>MSIISTKYLLQDAQANGYAVPAFNIHNAETIQAILEVCSEMRSPVILAGTPGTFKHIALEEIYALCSAYSTTYNMPLALHLDHHESLDDIRRKVHAGVRSAMIDGSHFPFAENVKLVKSVVDFCHSQDCSVEAELGRLGGVEDDMSVDAESAFL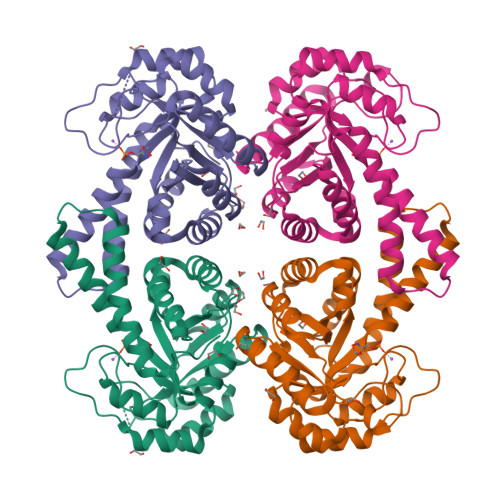TDPQEAKRFVELTGVDSLAVAIGTAHGLYSKTPKIDFQRLAEIREVVDVPLVLHGASDVPDEFVRRTIELGVTKVNVATELKIAFAGAVKAWFAENPQGNDPRYYMRVGMDAMKEVVRNKINVCGSANRISA[2x]> A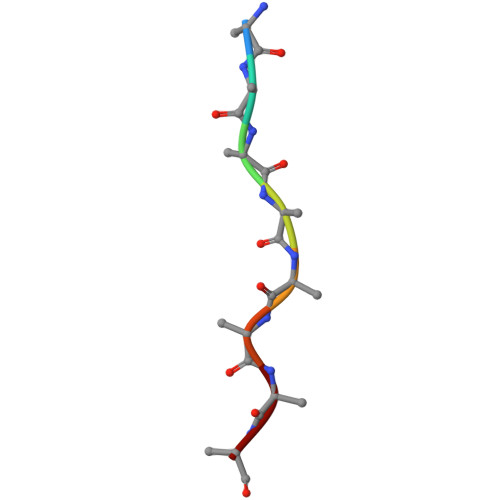AAAAAAA>MRGSHHHHHHGSMDKNIIIGAMTALITPFKNGKVDEQSYARLIKRQIENGIDAVVPVGTTGESATLTHEEHRTCIEIAVETCKGTKVKVLAGAGSAATHEAVGLAKFAKEHGADGILSVAPYYNKPTQQGLYEHYKAIAQSVDIPVLLYNVPGRTGCEISTDTIIKLFRDCENIYGVKEASGNIDKCVDLLAHEPRMMLISGEDAINYPILSNGGKGVISV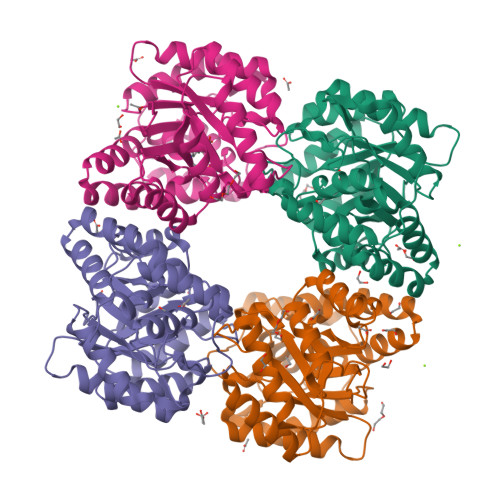TSNLLPDMISALTHFALDENYKEAKKINDELYNINKILFCESNPIPIKTAMYLAGLIESLEFRLPLCSPSKENFAKIEEVMKKYKIKGF[6x]>QHQKASNHSLHNLYNLQRDLLTVAATVLGKQDPVLTSMANQMELAKVKADRPATKQEEAAAKALKKNLIELIAARTQQQDGLPAKEAHRFAAVAFRDAQVKQLNNQPWQTIKNTLTHNGHHYTNTQLPAAEMKIGAKDIFPSAYEGKGVCSWDTKNIHHANNLWMSTVSVHEDGKDKTLFCGIRHGVLSPYHEKDPLLRHVGAENKAKEVLTAALFSKPELLNKALAGEAVSLKLVSVGLLTASNIFGKEGTMVEDQMRAWQSLTQPGKMIHLKIRNKDGDLQTVKIKPDVAAFNVGVNELALKLGFGLKASDSYNAEALHQLLGNDLRPEARPGGWVGEWLAQYP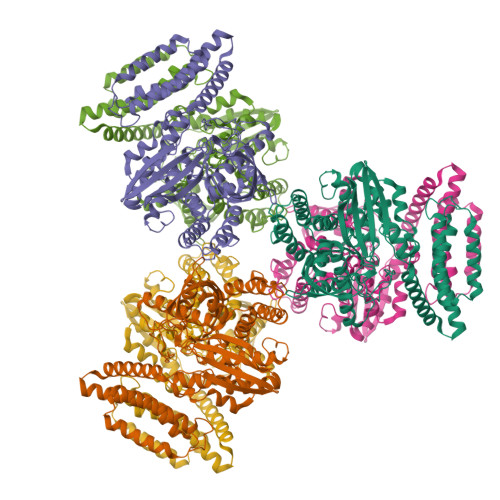DNYEVVNTLARQIKDIWKNNQHHKDGGEPYKLAQRLAMLAHEIDAVPAWNCKSGKDRTGMMDSEIKREIISLHQTHMLSAPGSLPDSGGQKIFQKVLLNSGNLEIQKQNTGGAGNKVMKNLSPEVLNLSYQKRVGDENIWQSVKGISSLITS[6x]> MGGKWSKSSIVGWPAIRERLRRAQPAAERRRAQPAAEGVGAASQDLGRHGALTSSNTDTTNADEEEEVGFPVRPQVPLRPMTYKGAVDLSFFLKEKGGLEGLVYSQREKEILDLWVYHTQGYFPDWQCYTPGPGVRYPLTFGWCFKLVPVDPGEVEEATEGENNCLLHPICQHGMDDDHREVLKWKFDSHLAHTHMARELHPEYFKNC;> MGGKWSKSSIVGWPAIRERLRRAQPAAERRRAQPAAEGVGAASQDLGRHGALTSSNTDTTNADEEEEVGFPVRPQVPLRPMTYKGAVDLSFFLKEKGGLEGLVYSQKRKEILDLWVYHTQGY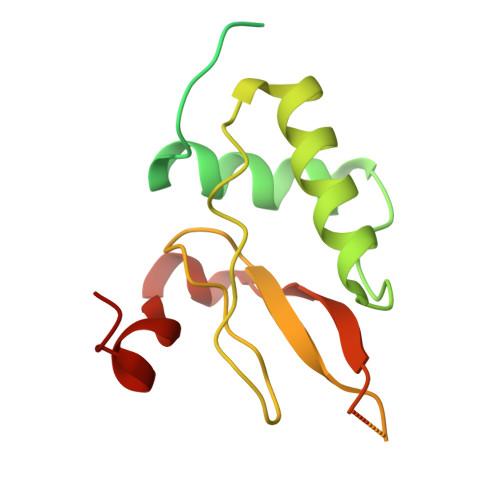FPDWQCYTPGPGVRYPLTFGWCFKLVPVDPGEVEEATEGENNCLLHPICQHGMDDDHREVLKWKFDSHLAHTHMARELHPEFYKNC3-IODO-BENZYL 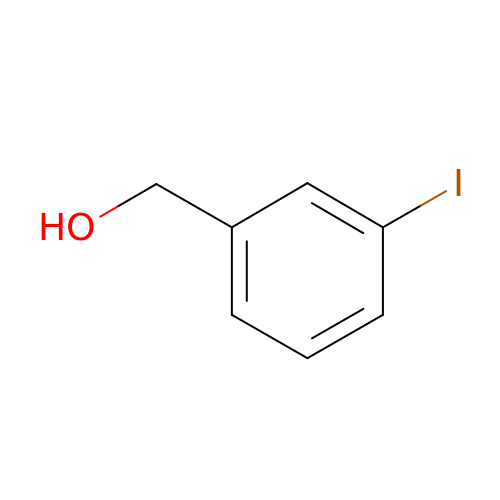ALCOHOL | C7 H7 I O | QGCCNWSXJHGUNL-UHFFFAOYSA-N> SMKITSSNFATIATSENFAKLSVLPKNHREPIKGLFKSAVEQFSSARDFFKNENYSKELAEKFNKEAVNEAVEKLQKAIDLAEK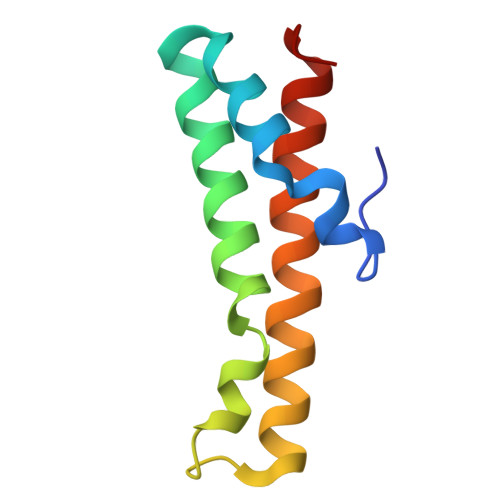QGIQF> MEFFGETWRRELAAEFEKPYFKQLMSFVADERSRHTVYPPADQVYSWTEMCDIQDVKVVILGQDPYHGPNQAHGLCFSVQKPVPPPPSLVNIYKELCTDIDGFKHPGHGDLSGWAKQGVLLLNAVLTVRAHQANSHKDRGWETFTDAVIKWLSVNREGVVFLLWGSYAHKKGATIDRKRHHVLQAVHPSPLSAHRGFLGCKHF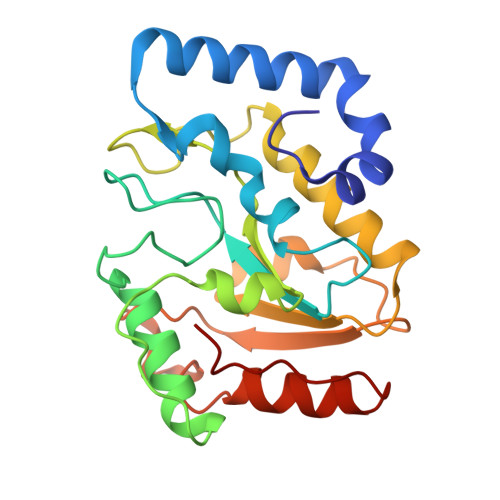SKANGLLKLSGTEPINWRAL>[3x]ATPHINAEMGDFADVVL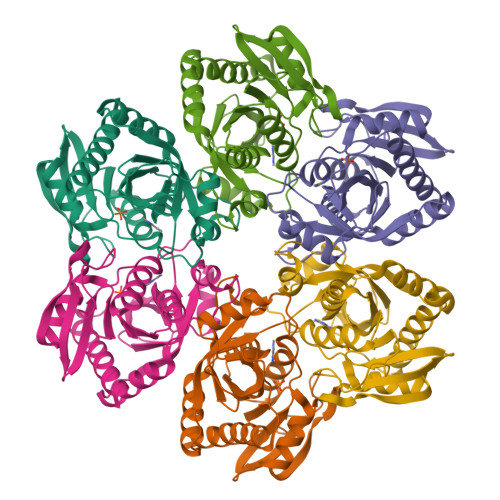MPGDPLRAKYIAETFLEDAREVNNVRGMLGFTGTYKGRKISVMGHGMGIPSCSIYTKELITDFGVKKIIRVGSCGAVLPHVKLRDVVIGMGACTDSKVNRIRFKDHDFAAIADFDMVRNAVDAAKALGIDARVGNLFSADLFYSPDGEMFDVMEKYGILGVEMEAAGIYGVAAEFGAKALTICTVSDHIRTHEQTTAAERQTTFNDMIKIALESVLLGDKE>[4x]MEHICGTSRIAGFRFSLYPMTDDFISVIKSALKKTDTSKVWTKTDHISTVLRGSIDHV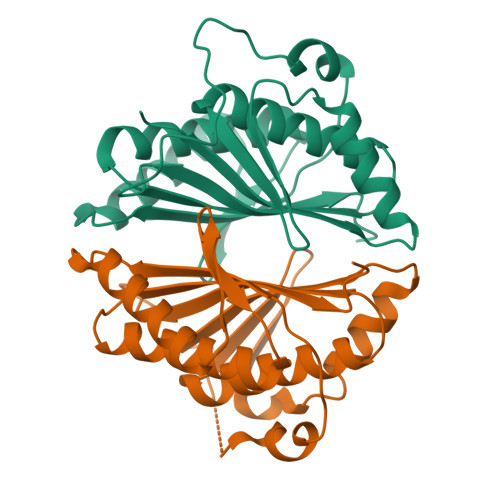FDAAKAIYLHAANSEQHIVMNGTFSIGCPGDTQGDTYLSKGDKRVNEDAVRGLKAEAPCQFALYPMNEPDYMGLIMEAVDIAKAQGTFVQGVHYASELDGDAHDVFSTLEAVFRMAEQQTNHITMTVNLSANSPSRKNRKQG>[2x]MASQPNSSAKKKEEKGKNIQVVVRCRPFNLAERKASAHSIVECDPVRKEVSVRTGGLADKSSRKTYTFDMVFGASTKQIDVYRSVVCPILDEVIMGYNCTIFAYGQTGTGKTFTMEGERSPNEEYTWEEVPLAGIIPRTLHQIFEKLTDNGTEFSVKVSLLEIYNEELFDLLNPSSDVSERLQMFDDPRNKR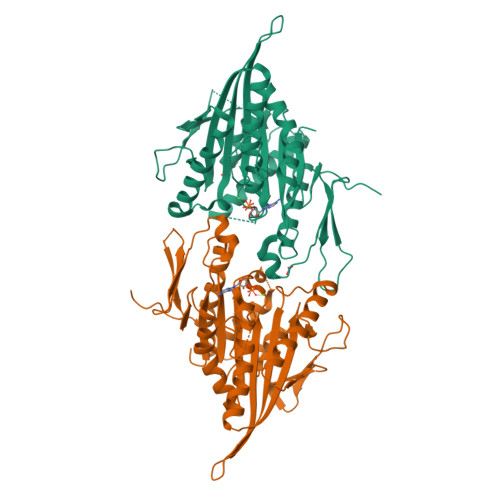GVIIKGLEEITVHNKDEVYQILEKGAAKRTTAATLMNAYSSRSHSVFSVTIHMKETTIDGEELVKIGKLNLVDLAGSENIGRSGAVDKRAREAGNINQSLLTLGRVITALVERTPHVPYRESKLTRILQDSLGGRTRTSIIATISPASLNLEETLSTLEYAHRAKNILNKPEVNQK> MRLWSWVLHLGLLSAALGCGLAERPRRARRDPRAGRPPRPAAGPATCATRAARGRRASPPPPPPPGGAWEAVRVPRRRQQREARGATEEPSPPSRALYFSGRGEQLRLRADLELPRDAFTLQVWLRAEGGQRSPAVITGLYDKCSYISRDRGWVVGIHTISDQDNKDPRYFFSLKTDRARQVTTINAHRSYLPGQWVYLAATYDGQFMKLYVNGAQVATSGEQVGGIFSPLTQKCKVLMLGGSALNHNYRGYIEHFSLWKVARTQREILSDMETHGAHTALPQLLLQENWDNVKHAWSPMKDGSSPKVEFSNAHGFLLDTSLEPPLCGQTLCDNTEVIASYNQLSSFRQPKVVRYRVVNLYEDDHKNPTVTREQVDFQHHQLAEAFKQYNISWELDVLEVSNSSLRRRLILANCDISKIGDENCDPECNHTLTGHDGGDCRHLRHPAFVKKQHNGVCDMDCNYERFNFDGGECCDPEITNVTQTCFDPDSPHRAYLDVNELKNILKLDGSTHLNIFFAKSSEEELAGVATWPWDKEALMHLGGIVLNPSFYGMPGHTHTMIHEIGHSLGLYHVFRGISEIQSCSDPCMETEPSFETGDLCNDTNPAPKHKSCGDPGPGNDTCGFHSFFNTPYNNFMSYADDDCTDSFTPNQVARMHCYLDLVYQGWQPSRKPAPVALAPQVLGHTTDSVTLEWFPPIDGHFFERELGSACHLCLEGRILVQYASNASSPMPCSPSGHWSPREAEGHPDVEQPCKSSVRTWSPNSAVNPHTVPPACPEPQGCYLELEFLYPLVPESLTIWVTFVSTDWDSSGAVNDIKLLAVSGKNISLGPQNVFCDVPLTIRLWDVGEEVYGIQIYTLDEHLEIDAAMLTSTADTPLCLQCKPLKYKVVRDPPLQMDVASILHLNRKFVDMDLNLGSVYQYWVITISGTEESEPSPAVTYIHGSGYCGDGIIQKDQGEQCDDMNKINGDGCSLFCRQEVSFNCIDEPSRCYFHDGDGVCEEFEQKTSIKDCGVYTPQGFLDQWASNASVSHQDQQCPGWVIIGQPAASQVCRTKVIDLSEGISQHAWYPCTISYPYSQLAQTTFWLRAYFSQPMVAAAVIVHLVTDGTYYGDQKQETISVQLLDTKDQSHDLGLHVLSCRNNPLIIPVVHDLSQPFYHSQAVRVSFSSPLVAISGVALRSFDNFDPVTLSSCQRGETYSPAEQSCVHFACEKTDCPELAVENASLNCSSSDRYHGAQCTVSCRTGYVLQIRRDDELIKSQTGPSVTVTCTEGKWNKQVACEPVDCSIPDHHQVYAASFSCPEGTTFGSQCSFQCRHPAQLKGNNSLLTCMEDGLWSFPEALCELMCLAPPPVPNADLQTARCRENKHKVGSFCKYKCKPGYHVPGSSRKSKKRAFKTQCTQDGSWQEGACVPVTCDPPPPKFHGLYQCTNGFQFNSECRIKCEDSDASQGLGSNVIHCRKDGTWNGSFHVCQEMQGQCSVPNELNSNLKLQCPDGYAIGSECATSCLDHNSESI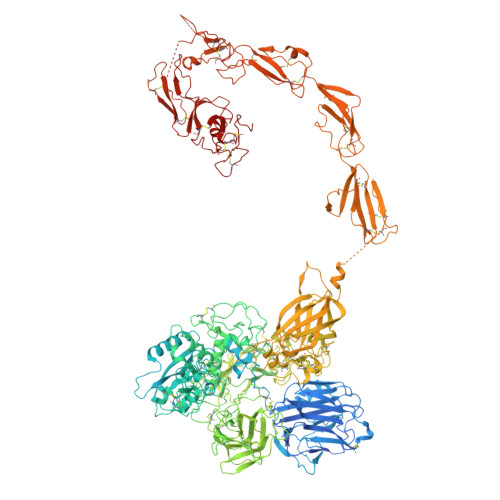ILPMNVTVRDIPHWLNPTRVERVVCTAGLKWYPHPALIHCVKGCEPFMGDNYCDAINNRAFCNYDGGDCCTSTVKTKKVTPFPMSCDLQGDCACRDPQAQEHSRKDLRGYSHG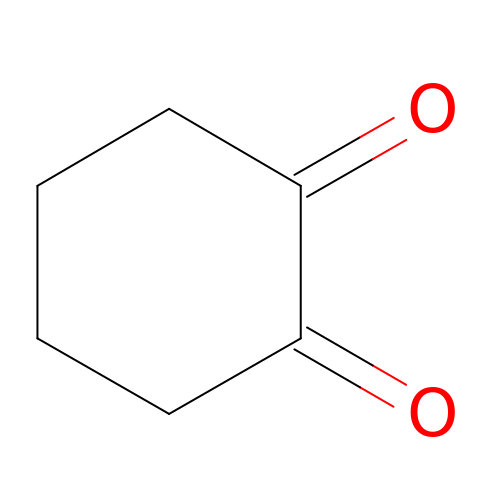CYCLOHEXANE-1,2-DIONE | C6 H8 O2 | OILAIQUEIWYQPH-UHFFFAOYSA-N>HHHHHHMFGQLTGGLEAAWSKLKGEEVLTKDNIAEPMRDIRRALLEADVSLPVVRRFVQSVSDQAVGMGVIRGVKPDQQLVKIVHDELVKLMGGEVSELQFAKSGPTVILLAGLQGVGKTTVCAKLACYLKKQGKSCMLIAGDVYRPAAIDQLVILGEQVGVPVYTAGTDVKPADIAKQGLK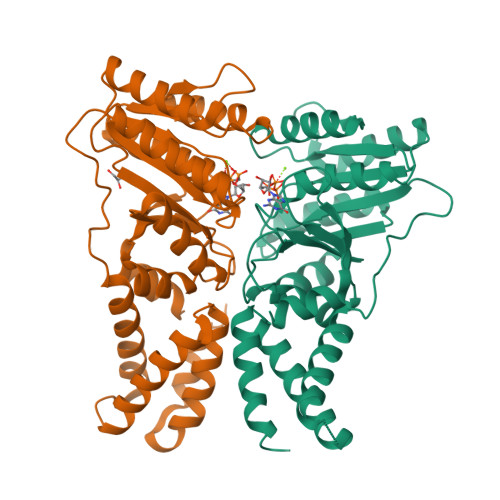EAKKNNVDVVIMDTAGRLQIDKGMMDELKDVKKFLNPTEVLLVVDAMTGQEAAALVTTFNVEIGITGAILTKLDGDSRGGAALSVKEVSGKPIKLVGRGERMEDLEPFYPDRMAGRILG[2x];>HHHHHHVIDELLLFWNLAETDRVLDELEEALLVSDFGPKITVRIVERLREDIMSGKLKSGSEIKDALKESVLEMLAKKNSKTELQLGFRKPAVIMIVGVNGGGKTTSLGKLAHRLKNEGTKVLMAAGDTFRAAASDQLEIWAERTGCEIVVAEGDKAKAATVLSKAVKRGKEEGYDVVLCDTSGRLHTNYSLMEELIACKKAVGKIVSGAPNEILLVLDGNTGLNMLPQAREFNEVVGITGLILTKLDGSARGGCVVSVVEELGIPVKFIGVGEAVEDLQPFDPEAFVNAIFS[2x]> SMPTDIEDINPNVYDRIKERVLTANEEDENVPDPFDKREIFDLIRNINDPEHPLTLEELHVVQEDLIRINDSQNSVHIS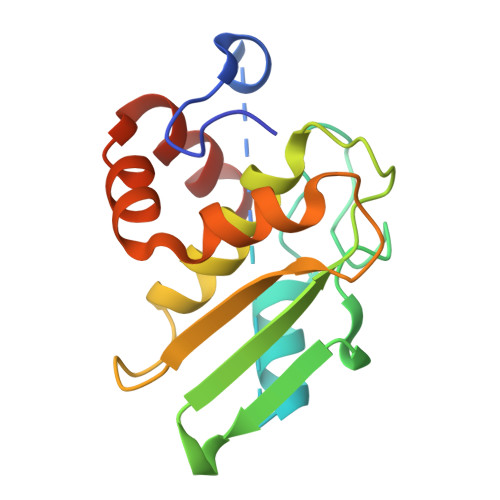FTPTIPHCSMATLIGLSIRVKLLRSLPPRFKVTVEITPGTHASELAVNKQLADKERVAAALENNHLAEVINQCIAAKG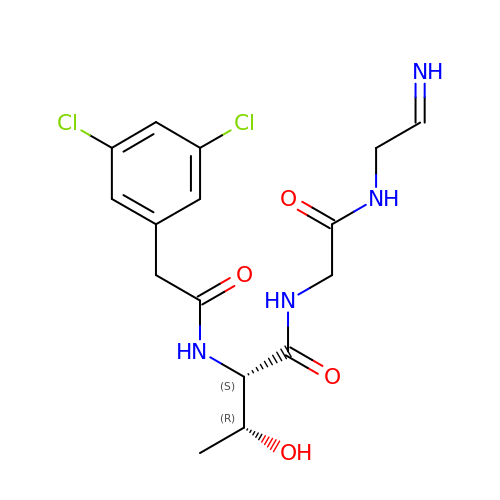N-[(3,5-dichlorophenyl)acetyl]-L-threonyl-N-[(2Z)-2-iminoethyl]glycinamide | C16 H20 Cl2 N4 O4 | MDMRSQQSLSAMBM-QMIWAGOPSA-N>MTTADLILINNWYVVAKVEDCRPGSITTAHLLGVKLVLWRSHEQNSPIQVWQDYCPHRGVPLSMGEVANNTLVCPYHGWRYNQAGKCVQIPAHPDMVPPASAQAKTYHCQERYGLVWVCLGNPVNDIPSFPEWDDPNYHKTYTKSYLIQASPFRVMDNSIDVSHFPFIHEGILGDRNHAEVEDLEVKVDKDGLTMGKYQVHTSKFNNSTKDDSMVNWFRLSHPLCQYCSTEASEMRTVDLMVVTPIDEDNSVLRYLIMWNGSKTLESKILADYDQVIEEDIRILHSQQPTRLP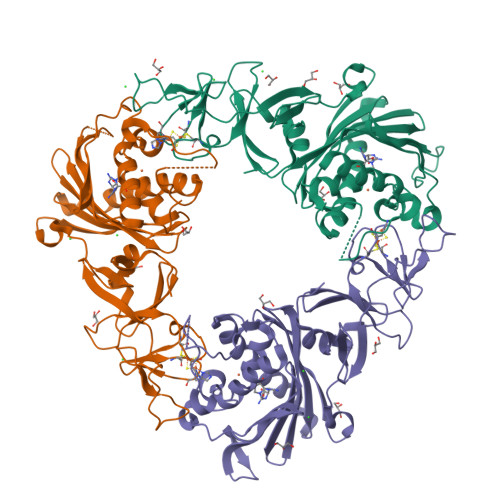LLSPKQINTQGLPQEIHVPSDRCTVAYRRWLKELGVTYGVC[3x]> YKPVIDWVKNRINARMRQYRKRSLKKKNHSKVIQRFKLTRFGW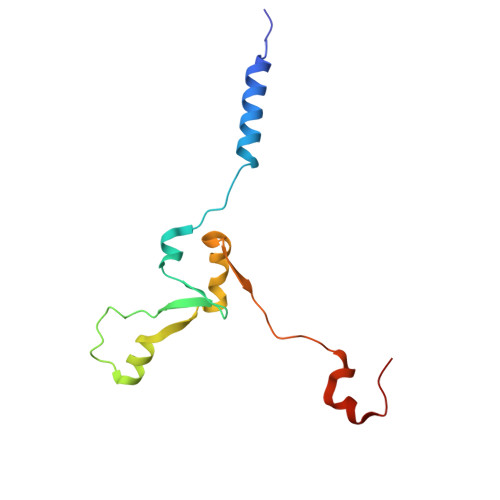QRLRSGRNGEKENLTHKQLKRTMGYTFVSRDDLWKFRFQLPSHILRLRDAPINRNPNIRKIRRSLPSYFG> SVLSDFQEAVPTVVGIPDGTAVVGRSFRVSIPTDLIASSGEIIKVSAAGKEALPSWLHWDPHSHILEGLPLDTDKGVHYISVSAARLGANGSHVPQTSSVFSIEVYPEDHNEPQSVHAASSDPGEVVPSACAADEPVTVLMVILDADLTKMTPKQRIDLLNRMQSFSEVELHNMKLVPVVNNRLFDMSAFMAGPGNAKKVVENGALLSWKLGCSLNQNSVPDIRGVETPAREGAMSAQLGYPVVGWHIANKKPTLPKRLRRQIH

Dystroglycan (DG) is composed of two subunits, α and β, that are formed from a unique precursor which undergoes a proteolytic event within the endoplasmic reticulum during the first steps of its maturation pathway. DG represents a widely expressed adhesion complex that plays a crucial role in offering stability to tissues, being at the crossroad between cytoskeleton, plasma membrane and the surrounding extracellular matrix. The DG main role is to bind with high-affinity laminins that are central organizers of the molecular network behind specialized basement membranes surrounding skeletal muscle. We have pioneered studies on α-DG at the molecular level, having extensively characterized the structure of its N-terminal domain, which is shaped in two subdomains.

Interestingly, the human T192M mutation (and its topological murine counterpart, T190M, which causes a similar dystrophic phenotype in a mouse model), lies within the strand B1 that together with the strands B2, B3, B4 and B5, arranged in an anti-parallel topology, defines the floor of the basket shaped S6-like domain. The crystal structure of T190M has been determined and refined up to a resolution of 1.6 Å. The overall structure of T190M does not show global differences with respect to WT. As reported for WT, the structure of T190M consists of two domains: the first one described as an Ig-like domain (residues 60–158) and the second one (residues 180–303) similar to the small subunit ribosomal protein S6. Despite showing very similar crystal structures, WT and T190M differ in the conformation of the flexible loop linking the two domains (residues 159–179). Moreover, in T190M the loop could be traced for three additional residues, up to Gln163, with respect to the WT structure, with residues (158–161) assuming a β-Turn structure. Despite the limited effect of the Thr to Met mutation on the neighboring residues, the introduction of a bulkier and apolar group such as the methylthio group of the methionine causes a re-organization of the surrounding water molecules. The lack of WAT304 in T190M is rather interesting, as this water molecule bridges together the B1 and B5 β-strands by interacting with the backbone of residues Val188 (O) and His296 (O), and with the side chains of residues Thr190 (Oγ1) and His296 (Nδ1). WAT304 acts as hydrogen bonds donor towards residues Val188 (O) and His296 (O) and as hydrogen bonds acceptor from Thr190 (Oγ1) and His296 (Nδ1). Such hydrogen bonds are not observed in T190M due to the lack of a bridging solvent molecule that would stabilize the interaction between the B1 and B5 β-strands. The plot of the emission spectra peaks as a function of GdnHCl reveals a cooperative unfolding behaviour for both WT and T190M, with transition midpoints (Gdn50%, i.e. the denaturant concentration inducing 50% of the total peak shift) of 1.45M and 1M, respectively, indicating that WT is more stable than T190M.> MWVYRLKGTLEALDPILPGLFDGGARGLWEREGEVWAFFPAPVDLPYEGVWEEVGDEDWLEAWRRDLKPALAPPFVVLAPWHTWEGAEIPLVIEPGMAFGTGHHETTRLALKALARHLRPGDKVLDLGTGSGVLAIAAEKLGGKALGVDIDPMVLPQAEANAKRNGVRPRFLEGSLEAALPFGPFDLLVANLYAELHAALAPRYREALVPGGRALLTGILKDRAPLVREAMAGAGFRPLEEAAEGEWVLLAYGR;> MKKVVA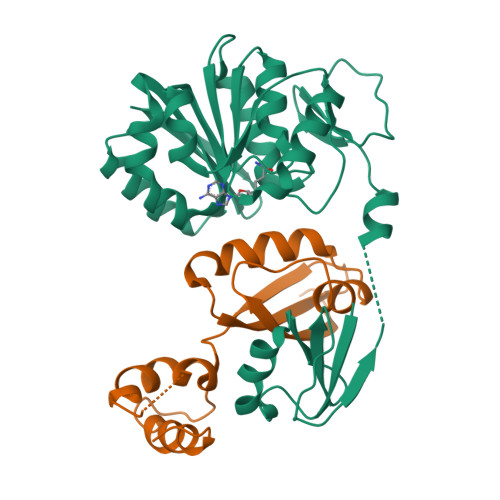VVKLQLPAGKATPAPPVGPALGQHGANIMEFVAAFNAATANMGDAIVPVEITIYADRSFTFVTKTPPASYLIRKAAGLEKGAHKPGREKVGRITWEQVLEIAKQKMPDLNTTDLEAAARMIAGSARSMGVEVVGAPEVKDA Deubiquitinating enzymes (DUBs) cleave peptide- and isopeptide-bonds downstream of ubiquitin. By performing a comprehensive bioinformatical screen, followed by biochemical and structural characterization of interesting candidates, we were able to identify active members of this family in a wide range of eukaryotic species and a few host-associated bacteria. Due to the similarity to the herpesvirus proteins, we refer to this extended enzyme family as VTD (for Viral Tegument-like Deubiquitinases). While some VTD activities resemble viral tegument DUBs in that they favor K48-linked ubiquitin chains, other members are highly specific for K6- or K63-linked ubiquitin chains.

To further elucidate the structural basis for VTD activity, we solved the crystal structure of DrT1-VTD2 (residues 300 to 520 of Uniprot entry A0A2R8QBC4) at a resolution of 1.90 Å and compared it to the ubiquitin complex of mouse cytomegalovirus M48, the only available structure of a herpesviral tegument deubiquitinase. The asymmetric unit contained one DrT1-VTD2 domain, which was completely resolved with the exception of residues 107 to 109 located in a protruding loop where Leu108 and Gly109 have rather weak density. In total, the structure contains four α-helices and nine β-strands, which adopt the form of an α-β-α sandwich, in which a bifurcated antiparallel β-sheet is flanked by α-helices. In VTDs, the catalytic histidine and aspartate residues form an invariable Asp-x-His motif, while in typical DUBs the catalytic Asp/Asn residue follows the His residue at a variable distance. As a consequence, the catalytic histidine (His453 in DrT1-VTD2 and His158 in M48) resides on the opposite site of the catalytic triad, creating a mirror image to the classic papain fold active site. To confirm the predicted role of Cys322, Asp451 and His453 as the catalytic triad of DrT1-VTD2, these residues were mutated to alanine and tested for their catalytic activity. Ubiquitin-AMC assays as well as incubation of K48-linked di-ubiquitin chains with C322A, D451A or H453A mutants demonstrated a complete loss of activity. When the DrT1-VTD2 residues 403–411 were replaced by a short Gly-Gly-Ser linker, the enzymatic activity against Ub-AMC and di-ubiquitin was completely lost. However, the quadruple mutant DrT1-VTD24mut (F398A, P405A, A406G and L407A) completely lost its activity against di-ubiquitin, suggesting a complex multi-factorial recognition of the ubiquitin Ile44 patch. Individual mutations of both residues (D376A and E377A) resulted in a strongly reduced chain cleaving activity, and also a reduced cleavage of Ub-AMC, the latter effect being more pronounced for E377A.

> GPLSVAASHCQSDVRYDSNSRNRQCTCNALMFLAVHNESNQLQSADLDCVLQKGDAVYSSVKRSLQNKGQFVHDFLNFDELPSTIETNSRCYNIVKHPQRFGFLKDTPALGEYQNLENTLQCLKSGLTDALLLCGGSCIAVFRDRTGRFGYFDSHSRTPDGKYTGEKSGTAVMLTFLHLKAMVEKLLQLFQGCLQLSDQEQFDLLPVSFIEIT> SQIPASEQETLVRPKPLLLKLLKSVGAQKDTYTMKEVLFYLGQYIMTKRLYDAAQQHIVYCSNDLLGDLFGVPSFSVKEHRKIYTMIYR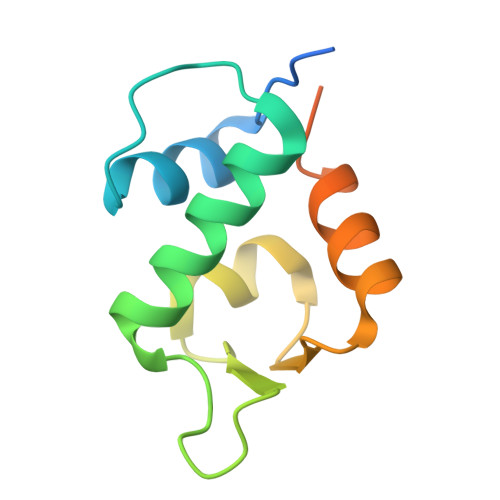NLVVVNQQESSDSGTSVSEN> MLNIQNYSASPHPGIVAERPQTPSASEHVETAVVPSTTEHRGTDIISLSQAATKIHQAQQTLQSTPPISEENNDERTLARQQLTSSLNALAKSGVSLSAEQNENLRSAFSAP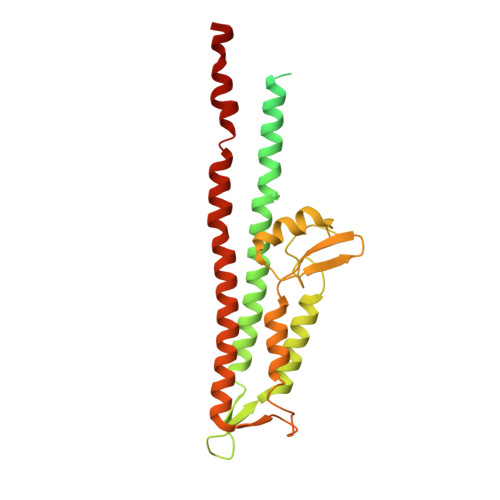TSALFSASPMAQPRTTISDAEIWDMVSQNISAIGDSYLGVYENVVAVYTDFYQAFSDILSKMGGWLLPGKDGNTVKLDVTSLKNDLNSLVNKYNQINSNTVLFPAQSGSGVKVATEAEARQWLSELNLPNSCLKSYGSGYVVTVDLTPLQKMVQDIDGLGAPGKDSKLEMDNAKYQAWQSGFKAQEENMKTTLQTLTQKYSNANSLYDNLVKVLSSTISSSLETAKSFLQG> AIGEFMVSLPRMVYPQPKVLTPCRKDVLVVTPWLAPIVWEGTFNIDILNEQFRLQNTTIGLTVFAIKKYVAFLKLFLETAEKHFMVGHRVHYYVFTDQPAAVPRVTLGTGRQLSVLEVRAYKRWQDVSMRRMEMISDFCERRFLSEVDYLVCVDVDMEFRDHVGVEILTPLFGTLHPGFYGSSREAFTYERRPQSQAYIPKDE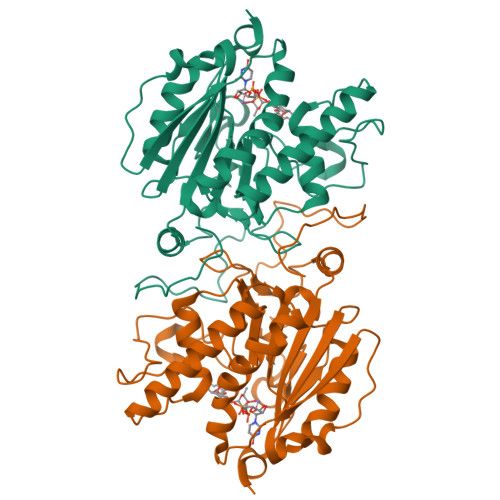GDFYYLGGFFGGSVQEVQRLTRACHQAMMVDQANGIEAVWHDESHLNKYLLRHKPTKVLSPEYLWDQQLLGWPAVLRKLRFTAVPKNHQAVRNPE> IIGGHEVTPHSRPYMASVRFGGQHHCGGFLLRARWVVSAAHCFSHRDLRTGLVVLGAHVLSTAEPTQQVFGIDALTTHPDYHPMTHANDICLLRLNGSAVLGPAVGLLRLPGRRARPPTAGTRCRVAGWGFVSDFEELPPGLME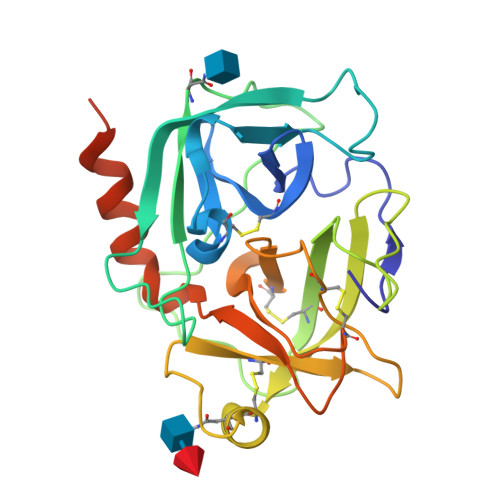AKVRVLDPDVCNSSWKGHLTLTMLCTRSGDSHRRGFCSADSGGPLVCRNRAHGLVSFSGLWCGDPKTPDVYTQVSAFVAWIWDVVRRSSPQPGPLPGTTRPPGEAA N-(4-phenoxyphenyl)-2-[(pyridin-4-ylmethyl)amino]nicotinamide 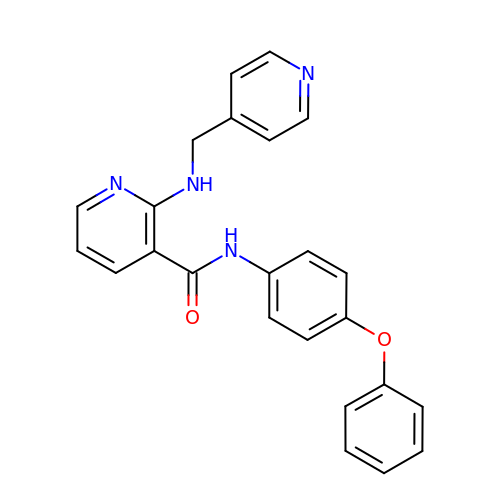| C24 H20 N4 O2 | CPVRYQAOUPSUDO-UHFFFAOYSA-N>MNELLHLAPNVWPRNTTRDEVGVVCIAGIPLTQLAQEYGTPLFVIDEDDFRSRCRETAAAFGSGANVHYAAKAFLCSEVARWISEEGLCLDVCTGGELAVALHASFPPERITLHGNNKSVSELTAAVKAGVGHIVVDSMTEIERLDAIAGEAGIVQDVLVRLTVGVEAHTHEFISTAHEDQKFGLSVASGAAMAAVRRVFATDHLRLVGLHSHIGSQIFDVDGFELAAHRVIGLLRDVVGEFGPEKTAQIATVDLGGGLGISYLPSDDPPPIAELAAKLGTIVSDESTAVGLPTPKLVVEPGRAIAGPGTITLYEVG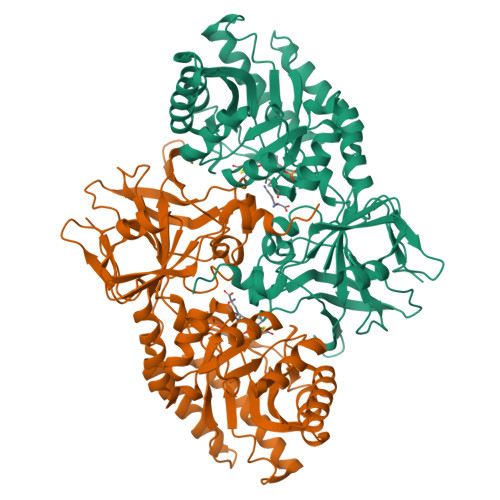TVKDVDVSATAHRRYVSVDGGMSDNIRTALYGAQYDVRLVSRVSDAPPVPARLVGKHCESGDIIVRDTWVPDDIRPGDLVAVAATGAYCYSLSSRYNMVGRPAVVAVHAGNARLVLRRETVDDLLSLEVRHHHHHH[2x]1-(2-bromo-4-chlorophenyl)-N-{(3S)-1-[(E)-iminomethyl]pyrrolidin-3-yl}methanesulfonamide 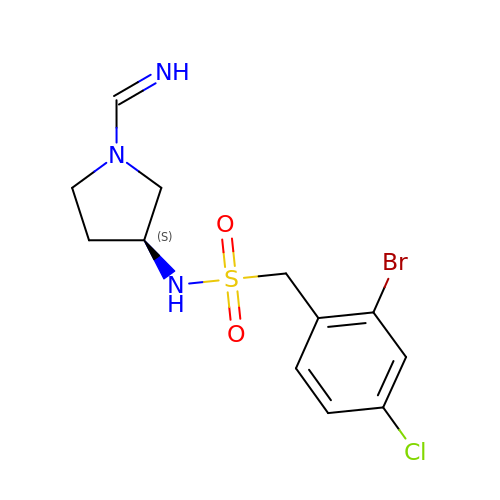| C12 H15 Br Cl N3 O2 S | JCYNDVNUPRPXTG-LWHXSLQUSA-N> MAENSEEDKQYLIFIKVFQQAMKGNFAKIYAKTEEGKDPPIKKKVERLRAELNYCYDELSFKEYLSDFLVRGGLNKYFNEHQEEIALLIKKSPWQEIRIWSLLAIASYKPKDKLTNRDDSSLSNNQK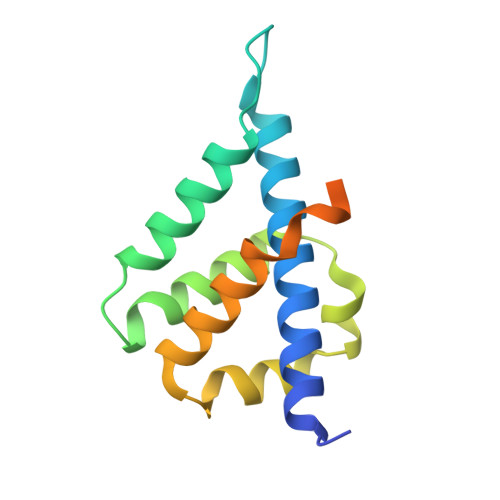LEEVNDDSEEE2,4-DIHYDROXYBENZOIC ACID | C7 H6 O4 | 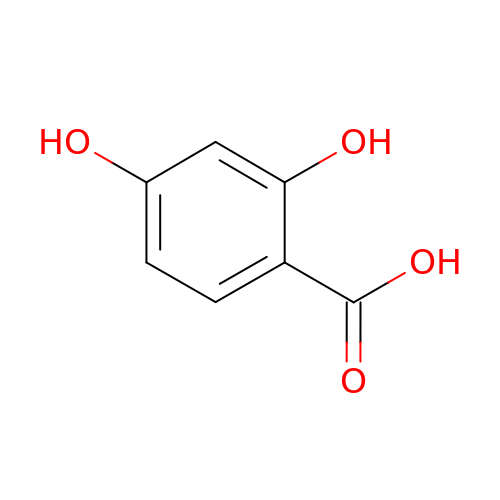UIAFKZKHHVMJGS-UHFFFAOYSA-N LANOSTEROL | C30 H50 O | 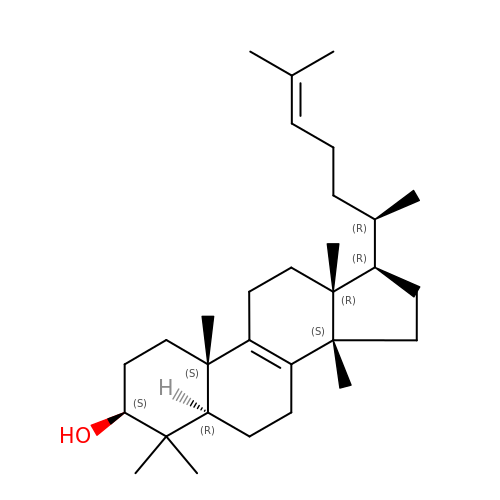CAHGCLMLTWQZNJ-BQNIITSRSA-N>GMTFRDTSAIASWHAHVYFDASSRDAAWTLREQIEAHWSGKLQLGRFHERPVGPHPMWSYQLAFTQEQFADLVGWLTLNH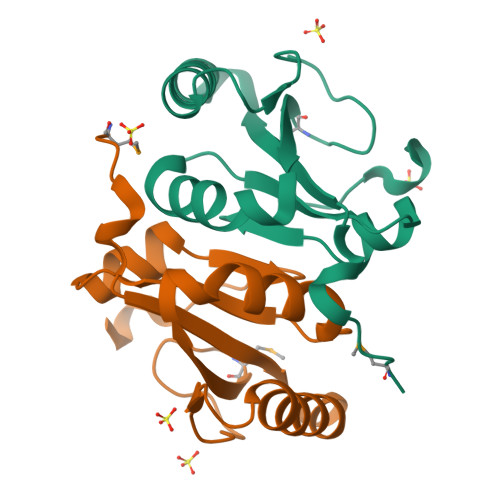GALDIFLHPNTGDALRDHRDAAVWIGHSHELVLSALN[2x]> MEITNVNEYEAIAKQKLPKMVYDYYASGAEDQWTLAENRNAFSRILFRPRILIDVTNIDMTTTILGFKISMPIMIAPTAMQKMAHPEGEYATARAASAAGTIMTLSSWATSSVEEVASTGPGIRFFQLYVYKDRNVVAQLVRRAERAGFKAIA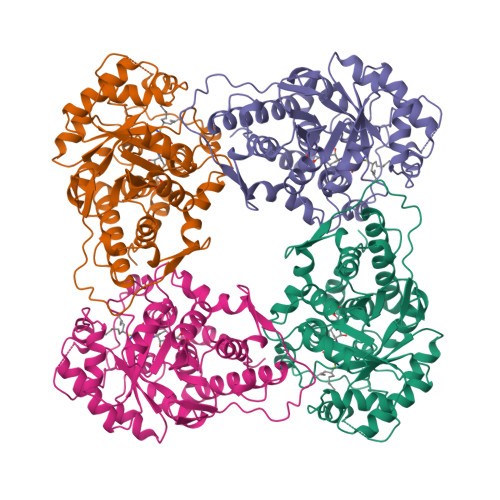LTVDTPRLGRREADIKNRFVLPPFLTLKNFEGIDLGKMDKANDSGLSSYVAGQIDRSLSWKDVAWLQTITSLPILVKGVITAEDARLAVQHGAAGIIVSNHGARQLDYVPATIMALEEVVKAAQGRIPVFLDGGVRRGTDVFKALALGAAGVFIGRPVVFSLAAEGEAGVKKVLQMMRDEFELTMALSGCRSLKEISRSHIAADWD4-[2-(propylamino)imidazo[2,1-b][1,3,4]thiadiazol-5-yl]phenol | C13 H14 N4 O S | 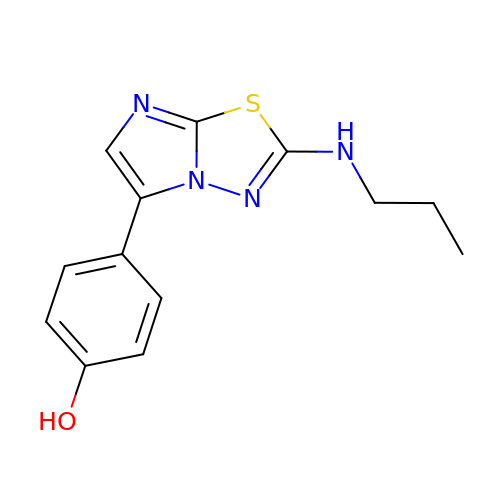CEHVGUOOKBVMCH-UHFFFAOYSA-N>MTNTTLDNNALDNNKLSPWPWQVDEAAISFDIESLGKKLKDLNQACYLINHAEKGLGIAQSAEVVGLAEPNNGLHPVSAFAPALGTQSLGDSNFRRVHGVKYAYYAGAMANGIASEELVIALGQAGILCSFGAAGLIPSRVEAAIKRIQAALPNGPYAFNLIHSPSEQALERGSVELFLKHQVRTVE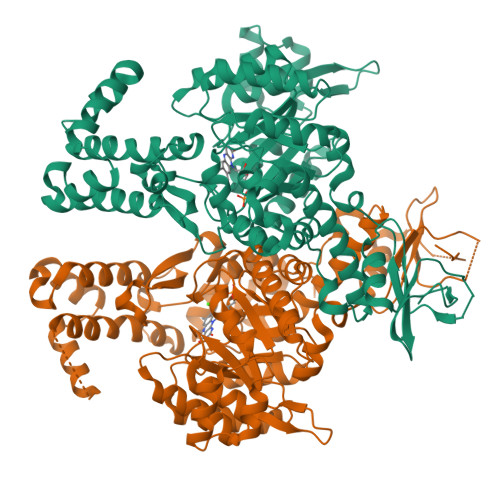ASAFLGLTPQIVYYRAAGLSRDASGEIVIGNKVIAKISRTEVATKFMEPAPVKILQQLVNEGLISEDQMLMAQSVPMADDITAEADSGGHTDNRPLVTLLPTILALKDTIQAKYQYKTPIRVGAGGGIGTPDAALATFNMGAAYIVTGSINQACVEAGASEHTRKLLATTEMADVTMAPAADMFEMGVKLQVVKRGTLFPMRANKLYEIYTRYDSIEAIPAEERQKLEEQVFRASLDEIWAGTVAHFNERDPKQIERALDNPKRKMALIFRWYLGLSSRWSNTGEVGREMDYQIWAGPALGAFNAWAKGSYLDDYRERNAVDLAKHLMQGAAYQARINLLLSQGVSIPVSLQRWKPLQRC[2x]>SMALSTQLIESVDKQSHLEEQLNKSLKTIASQKAAIENYNQLKEDYNTLKRELSDRDDEVKRLREDIAKENELR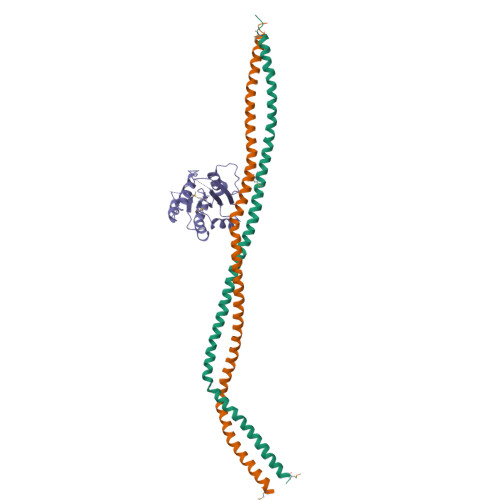TKAEEEADKLNKEVEDLTASLFDEANNMVADARKEKYAIEILNKRLTEQLREKDTLLDTLTLQLKNLKKVMHSLDNESTV[2x];> DSIMKILLIGDSGVGKSCLLVRFVEDKFNPSFITTIGIDFKIKTVDINGKKVKLQLWDTAGQERFRTITTAYYRGAMGIILVYDVTDERTFTNIKQWFKTVNEHANDEAQLLLVGNKSDMETRVVTADQGEALAKELGIPFIESSAKNDDNVNEIFFTLAKLIQEKIDSN> MPMQMFMQVYDEIQMFLLEELELKFDMDPNRVRYLRKMMDTTCLGGKYNRGLTVIDVAESLL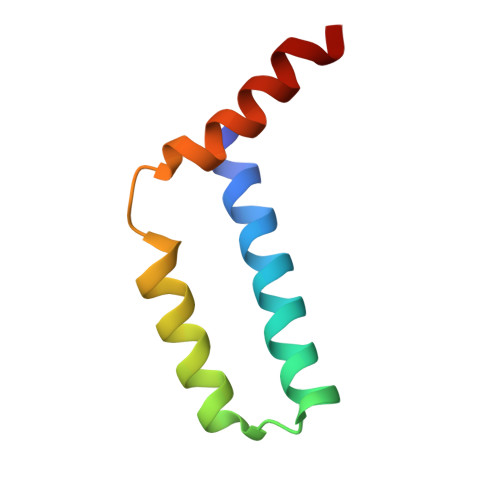S>[8x]MHHHHHHGSNKKSLSVIFVKPPFQLKKKFQKDPFYEIEMRKQLQMQQDGINNMTIFEWLKNRENFKKYGRNPKSKKIQEDFRDRYRNAKIDEYLLLYEDMDIKAIEAMVDSELEGLAALANPAQIAGGYVDVVTQMGNKRINSSIGSQWGSIEKGRSLNIENELLKLITDPPPITEEEQKKIKMNVNLVENLEIVK

We identify a horizontally transferred T6SS with Ntox15 family nuclease effector (Tde1) that mediates interbacterial antagonism among Bacteroidales, including several derived from a single human donor. Effectors with novel toxin 15 (Ntox15) DNAse domains, also known as toxin_43 domains, degrade recipient genomic DNA. Cognate immunity proteins are encoded adjacent to T6SS effectors and neutralize their activity to prevent intoxication of self and kin. Crystallographic snapshots of isolated Tde1, the Tde1/Tdi1 complex, and homologs from Phocaeicola vulgatus (Tde2/Tdi2) illustrate a conserved mechanism of immunity inserting into the central core of Tde, splitting the nuclease fold into two subdomains.

Tde1tox exhibited DNAse activity on plasmid dsDNA, which was abrogated by mutation of the HxxD active site (H279A) and strongly inhibited by the presence of Tdi1 or chelation of divalent cations using EDTA. A structural model of Tde1tox H279A/D282A Ntox15 domain was obtained by X-ray crystallography with diffraction data extending to 2.9 Å resolution. Although no close homologs of known structure were available, phases were solved by molecular replacement using an AlphaFold2 prediction model. The AlphaFold2 prediction model was very similar to the experimental crystal structure; mean Cα r.m.s.d. among the eight monomers in the asymmetric unit was 1.0 Å. The Ntox15 domain adopts a globular fold which is predominantly α-helical, forming a short α-sheet between helices 5 and 6 immediately adjacent to the active site. A cavity adjacent to the mutated HxxD motif marks the active site. A sulfate ion is modeled within the active site, likely an artifact of crystallization in high concentration of ammonium sulfate. The DNA binding site predicted with ProNA2020 (38) maps to helices 4, 6, and 7, adjacent to the active site. Coulombic surface rendering highlights relative positive surface charge surrounding the active site pocket, consistent with favorable electrostatics for interaction with negatively charged DNA. We conclude that Ntox15 domains adopt a globular fold, distinct from other nuclease families of known structure, with a structurally well-defined active site that mediates DNAse activity.> MNSPPSFGVNMTLVTLPEDLPVGAVAFWLVATDSDNDHLTYGISGPNASYFSVNANTGEVKLASPLDFETVPFFKITISTSDGLNIRTAEMQVIVEDRNDNIPVFLNTEFSTSINETLPVGSVVFSVLAEDKDTGTAGLVQYFIEKVIPSTANSNNLFRILENGSIVLNDTLSYNNKSAFYQLELKACDSGGILDNKPKTQCSQPVFVSISVIDEPDLDPRFIREFYSASVAEDATLGTSVLTVEAVDSDKGINDIVTYSVSNSTRPGWFDIREDGVIFVNGSLDREQLLLENEEVQIQVTATEKNLNIYGQEAKAS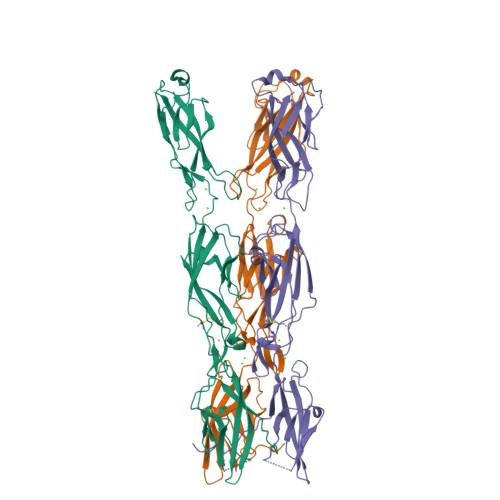MWVTIRVTDVNDLEHHHHHH> MARPNFRYTHYDLKELRAGTTLEISLSSVNNVRLMTGANFQRFTELLDFKYLGGVAKKSPIRIAVPETMHWHLIIDAEGHSGLAESSVK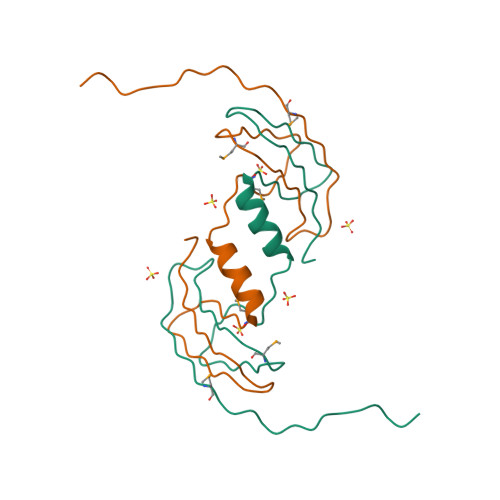MLPAQPQATLTRKAS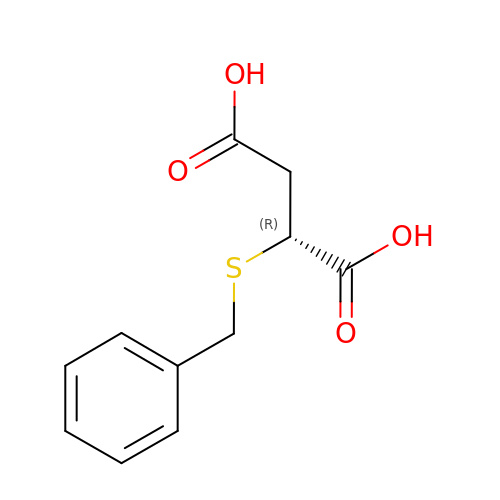(2~{R})-2-(phenylmethylsulfanyl)butanedioic acid | C11 H12 O4 S | PLQQDQFONINWJP-SECBINFHSA-N>[4x]MAHHHHHHMPGSELISGGWFREENDQWPGQAMSLRVEKVLYDAPTKFQHLTIFESDPKGPWGTVMALDGCIQVTDYDEFVYHEVLGHTSLCSHPKPERVLIIGGGDGGVLREVLRHGTVEHCDLVDIDGEVMEQSKQHFPQISRSLADPRATVRVGDGLAFVRQTPDNTYDVVIIDTTDPAGPASKLFGEAFYKDVLRILKPDGICCNQGESIWLDLELIEKMSRFIRETGFASVQYALMHVPTYPCGSIGTLVCSKKAGVDVTKPLRPVEDMPFAKDLKYYDSEMHKASFALPRFARHINNSE

In this study, to demonstrate the utility of virtual screening with protein dynamics, MD simulations were performed on Trypanosoma cruzi spermidine synthase to obtain an ensemble of dominant binding sites with a high probability of existence. The structure of the binding site obtained through MD simulation revealed pockets in addition to the active site that was present in the initial structure. Using the obtained binding site structures, virtual screening of 4.8 million compounds by docking simulation, in vitro assays, and X-ray analysis was conducted, successfully identifying two hit compounds.

As a result, TcSpdSyn IC50 values for two compounds were determined, with compounds 1 and 2 inhibiting TcSpdSyn at IC50 values of 82.27 and 43.41 μM, respectively. To examine the binding sites used by these two active compounds, we conducted X-ray crystallographic analyses to observe the structures of the TcSpdSyn complex with the two top-ranked compounds (compounds 1 and 2) in the hidden binding pocket, as predicted by the MD simulations. Compound 2 interacts with Glu22 and Asp77, similar to 1, and the lone pair of the quinoline nitrogen atom in 2 is proximal to the carboxylate group of Glu22. Thus, these results suggest that Glu22 is in a neutral state when interacting with the lone pair of quinoline. Compound 2 interacted with Glu22 and Asp77 (interaction energy values: −20.08 and −30.05 kcal/mol, respectively) through two hydrogen bonds in the same manner as 1. In particular, Asp77 interacted with compound 2 in a neutral state. Moreover, some weak interactions, such as with Ile71 Tyr245 and Ile247, were confirmed, with interaction energy values of −7.16, −6.96, and −5.71 kcal/mol, respectively. Comparing the structures of compounds 1 and 2, both are para-substituted anisoles with nitrogen-rich heterocycle para-substituents. However, the X-ray structures display opposite orientations for compounds 1 and 2 at the new site. Compound 1 interacts with Glu22 through the hydroxy group at the meta-position of anisoles, while compound 2 interacts with Glu22 via a secondary amine at para-substituent.>SNAYPDLAPP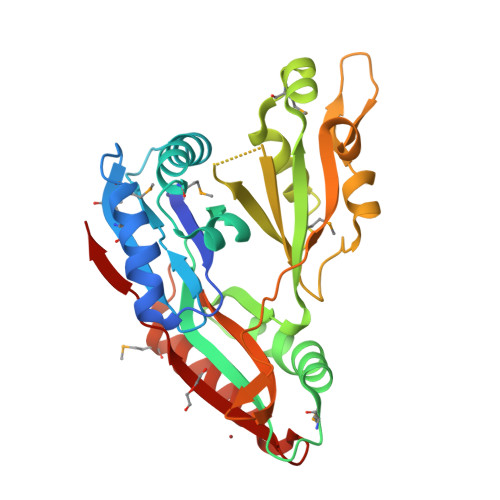NVRITANYPGASAQTLENTVTQVIEQNMTGLDNLMYMSSQSSGTGQATITLSFIAGTDPDEAVQQVQNQLQSAMRKLPQAVQDQGVTVRKTGDTNILTIAFVSTDGSMDKQDIADYVASNIQDPLSRVNGVGDIDAYGSQYSMRIWLDPAKLNSFQMTTKDVTDAIESQNAQIAVGQLGGTPSVDKQALNATINAQSLLQTPQQFRDITLRVNQDGSEVKLGDVATVELGAEKYDYLSRFNGNPASGLGVKLASGANEMATAKLVLDRLNELAQYFPHGLEYKIAYETTSFVKA[2x]>[2x]GAMDEKFIRETIETRIMMEVFCLENYFDKIAGS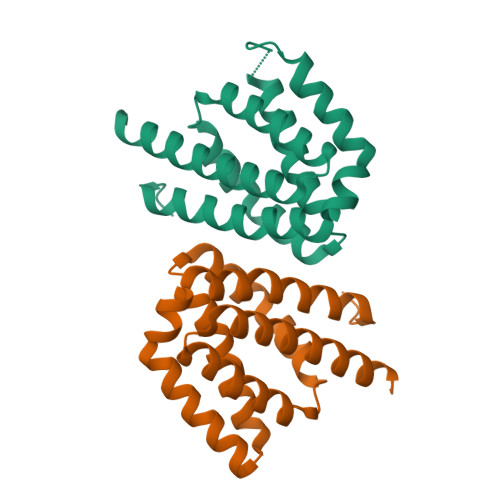EELLEIKGEIDDVEKSAKREIFDDSDERLHKLFIRASGNELIISLYEKIWDRIDLVRHLNERYVVSNREHKELIERIISGDKEGAIEKLKEHLKNVEAETIKNLYTY>MVSRYVPDM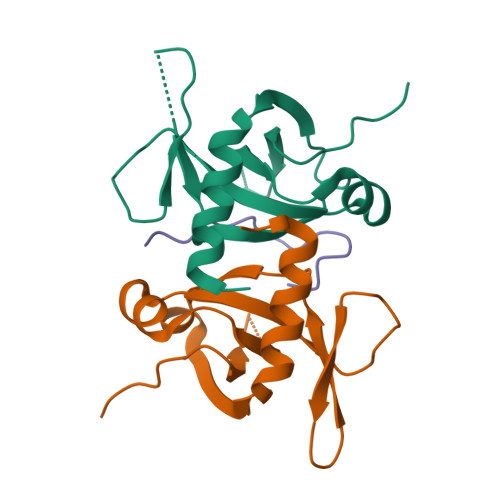GDLIWVDFDPTKGSAQAGHRPAVVLSPFMYNNKTGMCLCVPCTTQSKGYPFEVVLSGQERDGVALADQVKSIAWRARGATKKGTVAPEELQLIKAKINVLIGLSHHHHHH[2x];> HENIDWGEPKDKEVW> MNQIDLNVTCRYAGVFHVEKNGRYSISRTEAADLCQAFNSTLPTMDQMKLALSKGFETCRYGFIEGNVVIPRIHPNAICAANHTGVYILVTSNTSHY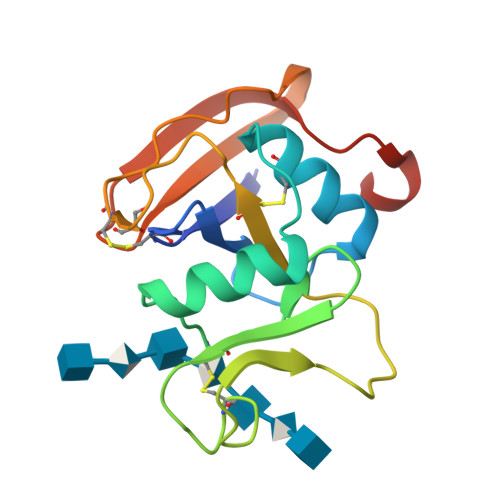DTYCFNASAPPEEDCTSVTDLPNSFDGPVTITIVNRDGTRYSKKGEYRTHQEDIDAS>MMQISSNGITRLKREEGERLKAYSDSRGIPTIGVGHTGKVDGNSVA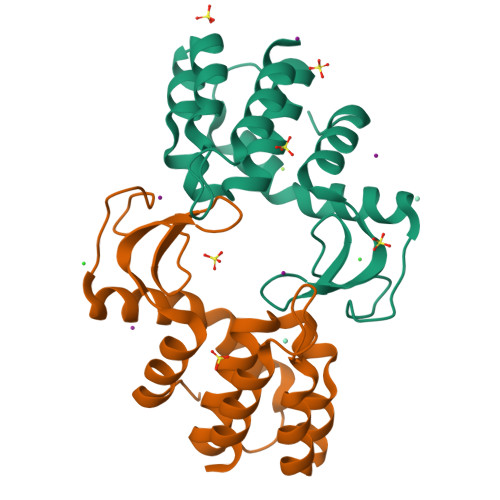SGMTITAEKSSELLKEDLQWVEDAISSLVRVPLNQNQYDAMCSLIFNIGKSAFAGSTVLRQLNLKNYQAAADAFLLWKKAGKDPDILLPRRRRERALFLS[2x]5-(2,6-diethylphenyl)thiophene-2-carboxylic 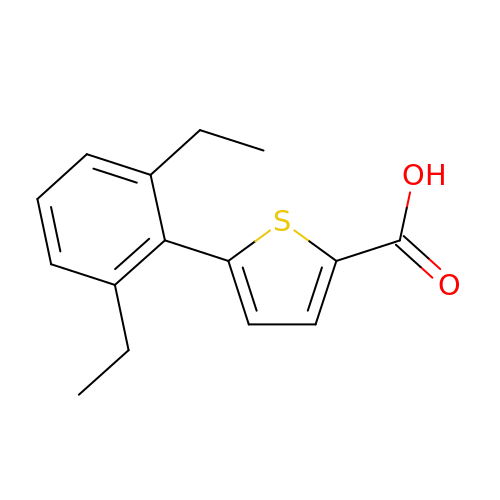acid | C15 H16 O2 S | OZTRYCWXRAYPCS-UHFFFAOYSA-N>ASMTGGQQMGRILVAVLISGTGSNLQALIDSTREPNSSAQIDIVISNKAAVAGLDKAERAGIPTRVINHKLYKNRVEFDSAIDLVLEEFSIDIVCLAGFMRILSGPFVQKWNGKMLNIHPSL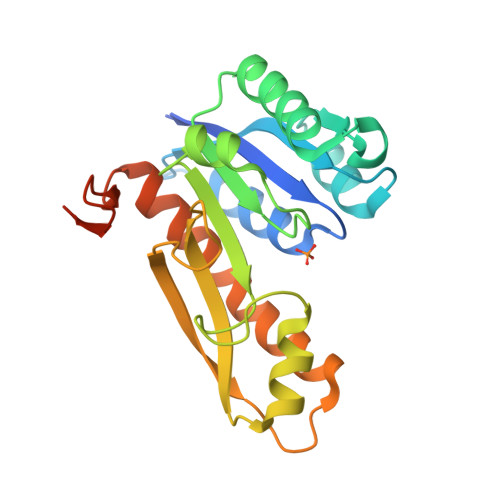LPSFKGSNAHEQALETGVTVTGCTVHFVAEDVDAGQIILQEAVPVKRGDTVATLSERVKLAEHKIFPAALQLVASGTVQLGENGKICWVKEEPLEHHHHHH[3x]> NIYQFKNMIECTVPARSWWDFADYGCYCGGGGSGTPTDDLDRCCQVHDNCYNQ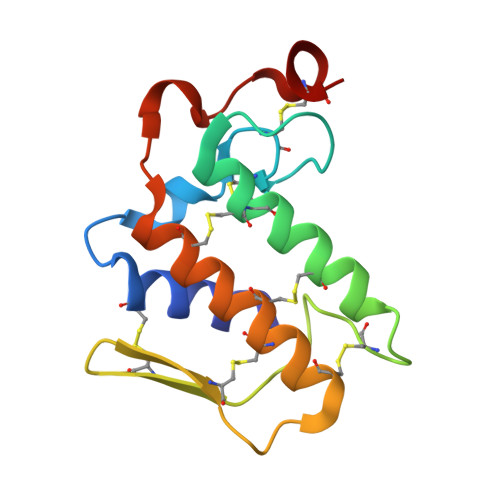AQEITGCRPKWKTYTYQCTQGTLTCKGRNNACAATTCDCDRLAAICFAGAPYNDTNYNIDLKARCQ> MALHTQVVDHYENPRNVGSLDKTSKNVGTGLVGAPACGDVMKLQIQVDEKGKIVDARFKTFGCGSAIASSSLATEWVKGKTVEEAL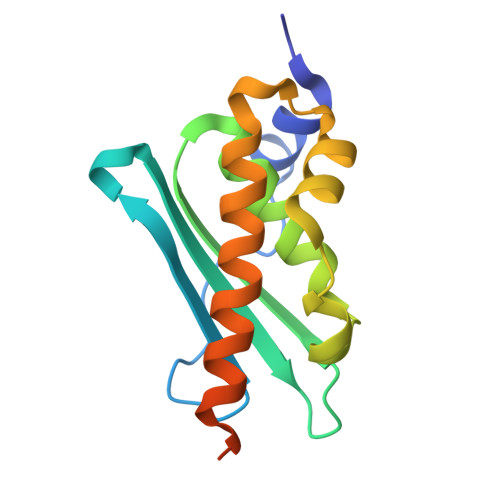TIKNTDIAKELCLPPVKLHCSMLAEDAIKAALADYKLKQEPKKGEAEKKLEHHHHHH> IGWRREGIKYRRNELFLDVLESVNLLMSPQGQVLSAHVSGRVVMKSYLSGMPECKFGMNDKIVIEKQGKGTADETSKSMEQKLISEEDLGKQSIAIDDCTFHQCVRLSKFDSERSISFIPPDGEFELMRYRTTKDIILPFRVIPLVREVGRTKLEVKVVIKSNFKPSLLAQKIEVRIPTPLNTSGVQVICMKGKAKYKASENAIVWKIKRMAGMKESQISAEI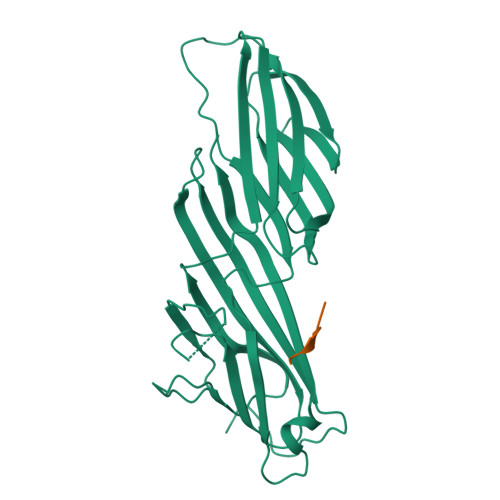ELLPTNDKKKWARPPISMNFEVPFAPSGLKVRYLKVFEPKLNYSDHDVIKWVRYIGRSGIYETRC;> QYKSILQE>MGPLPVCLPIMLLLLLPSLLLLLLLPGPGSGEASRILRVHRRGILELAGTVGCVGPRTPIAYMKYGCFCGLGGHGQPRDAIDWCCHGHDCCYTRAEEAGCSPKT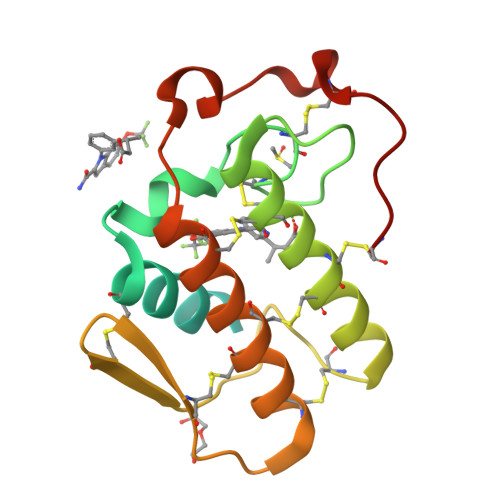ERYSWQCVNQSVLCGPAENKCQELLCKCDQEIANCLAQTEYNLKYLFYPQFLCEPDSPKCD[2x]Class Ia ribonucleotide reductases (RNRs) are allosterically regulated by ATP and dATP to maintain the appropriate deoxyribonucleotide levels inside the cell for DNA biosynthesis and repair. The α2 subunit houses the active site and the allosteric sites, and the β2 subunit houses the di-iron-tyrosyl radical cofactor.3−6 On every round of turnover, these subunits come together to form an active α2β2 complex, which allows for the transfer of the radical species from β to α, affording ribonucleoside diphosphate reduction. Excess dATP inhibits RNR through the creation of an α–β interface that restricts the ability of β2 to obtain a position that is capable of radical transfer. ATP breaks the α–β interface, freeing β2 and restoring enzyme activity.

We reasoned that substitutions of either F87 or W28 with Ala would create room for ATP binding in site 2 regardless of the position of H59 and thus be independent of the presence of ATP in site 1. We also confirmed that W28A substitution does not alter ATP binding in site 2 by determining a crystal structure of W28A α2 with ATP as the only effector at 2.6-Å resolution. We find that the W28A substitution results in a more open pocket for ATP binding at site 2, but no structural perturbations in the bound ATP molecule are apparent. All site 1 residues and site 2 residues F87 and F97 adopt analogous positions to those found in wild-type α2-(ATP)2. Therefore, the W28A substitution appears successful in uncoupling nucleotide binding in site 2 from the identity of the nucleotide in site 1 without substantially altering ATP binding to site 2. Although not the focus of this report, the W28A α2-(ATP)2/CDP structure at 2.6-Å resolution also provides a higher-resolution picture of the active site bound to the CDP/ATP substrate/effector pair. The hydrogen-bonding pattern that affords substrate specificity is the same as that described previously.

>[8x]MGSSHHHHHHSSGLVPRGSMNQNLLVTKRDGSTERINLDKIHRVLDAAAEGLHNVSISQVELRSHIQFYDGIKTSDIHETIIKAAADLISRDAPDYQYLAARLAIFHLRKKAYGQFEPPALYDHVVKMVEMGKYDNHLLEDYTEEEFKQMDTFIDHDRDMTFSYAAVKQLEGKYLVQNRVTGEIYESAQFLYILVAACLFSNYPRETRLQYVKRFYDAVSTFKISLPTPIMSGVRTPTRQFSSCVLIECGDSLDSINATSSAIVKYVSQRAGIGINAGRIRALGSPIRGGEAFHTGCIPFYKHFQTAVKSCSQGGVRGGAATLFYPMWHLEVESLLVLKNNRGVEGNRVRHMDYGVQINKLMYTRLLKGEDITLFSPSDVPGLYDAFFADQEEFERLYTKYEKDDSIRKQRVKAVELFSLMMQERASTGRIYIQNVDHCNTHSPFDPAIAPVRQSNLCLEIALPTKPLNDVNDENGEIALCTLSAFNLGAINNLDELEELAILAVRALDALLDYQDYPIPAAKRGAMGRRTLGIGVINFAYYLAKHGKRYSDGSANNLTHKTFEAIQYYLLKASNELAKEQGACPWFNETTYAKGILPIDTYKKDLDTIANEPLHYDWEALRESIKTHGLRNSTLSALMPSETSSQISNATNGIEPPRGYVSIKASKDGILRQVVPDYEHLHDAYELLWEMPGNDGYLQLVGIMQKFIDQSISANTNYDPSRFPSGKVPMQQLLKDLLTAYKFGVKTLYYQNTRDGAEDAQDDLVPSIQDDGCESGACK>[6x]MLMRTDPFRDLDR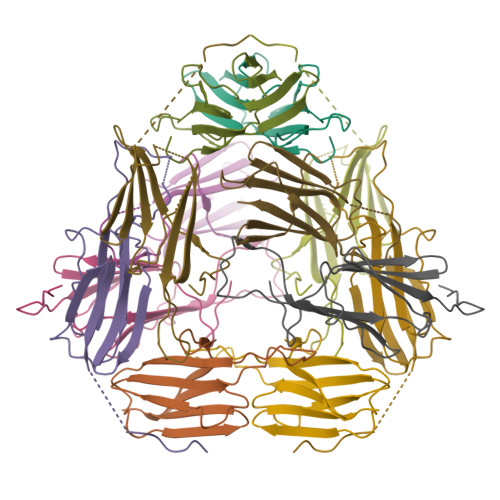FAQQVLGTSARPAVMPMDAWREGDKFVVEFDLPGIDADSLDIDIERNVVTVRAERPAVDPNREMLASERPRGVFSRQLVLGENLDTARIAASYTEGVLKLQIPVAEKAKPRKISITRGAGDKTISENGAHPEVIEA>[2x]MLKKILLLALLPAIAFAEELPAPVKAIEKQGITIIKTF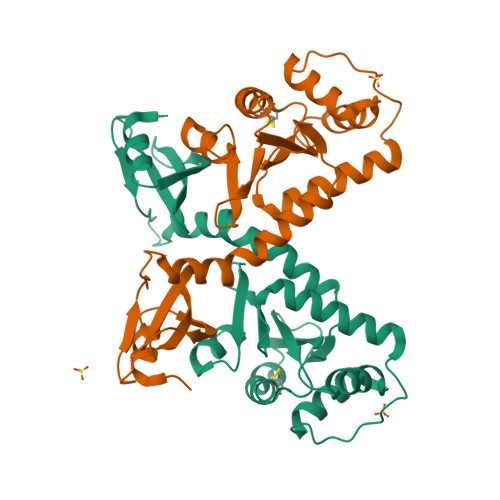DAPGGMKGYLGKYQDMGVTIYLTPDGKHAISGYMYNEKGENLSNTLIEKEIYAPAGREMWQRMEQSHWLLDGKKDAPVIVYVFADPFCGPCKQFWQQARPWVDSGKVQLRTLLVGVIKPESPATAAAILASKDPAKTWQQYEASGGKLKLNVPANVSTEQMKVLSDNEKLMDDLGANVMPAIYYMSKENTLQQAVGLPDQKTLNIIMGNKTRHHHHHH>ATSSTAVGFDERMLLHSEFEVKAQPHPERPDRLRAIAASLATAGVFPGRCLPINAREITKQELQMVHTSEHVDAVDTTSQLLYSYFTSDTYANEYSARAARLAAGLCADLATDIFTGRVKNGFALVRPPGHHAGVRHAMGFCLHNNAAVAALVAQAAGAKKVLIVDWDVHHGNGTQEIFEQNKSVLYISLHRHEGGNFYPGTGAADEVGSNGGEGYCVNVPWSCGGVGDKDYIFAFQHVVLPIASAFSPDFVIISAGFDAARGDPLGCCDVTPAGYSRMTQMLGDLCGGKMLVILEGGYNLRSISASATAVIKVLLGENPENELPIATTPSVAGLQTVLDVLNIQLEFWPSLAISYSKLLSEL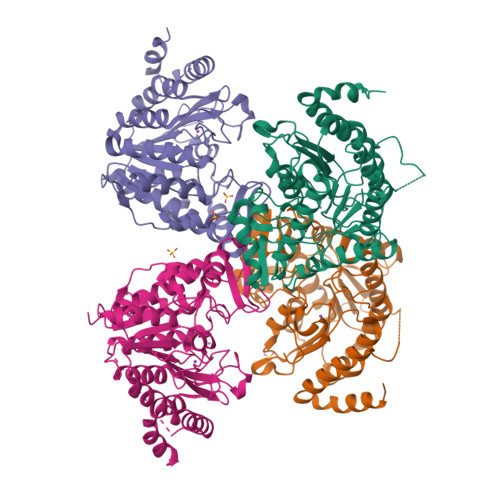E[4x]>AMADYDTYVSNVQINNLSYGVYTSGGKETQFFCIGLKHGSEAISINAMCKVDVYGNHKQGFDNMLNTAKYYYTTGGDVRIYYKENVWRDPDFKSAFSSRELIAITTCSSSSYCMGPTVTN[5x];> NISDYKVMTWNLQGSSASTESKWNVNVRQLLSGTAGVDILMVQEAGAVPTSAVPTGRHIQPFGVGIPIDEYTWNLGTTSRQDIRYIYHSAIDVGARRVNLAIVSRQRADNVYVLRPTTVASRPVIGIGLGNDVFLTAHALASGGPDAAAIVRVTINFFRQPQMRHLSWFLAGDFNRSPDRLENDLMTEHLERVVAVLAPTEPTQIGGGILDYGVIVDRAPYSQRVEALRNPQLASDHYPVAFLARSCL;> VDFVYRVDSTPPDVIFRDGFSLLGYNRNFQQFISGRSCSGGSSDSRYIATTSSVNQTYAIARAYYSRSTFKGNLYRY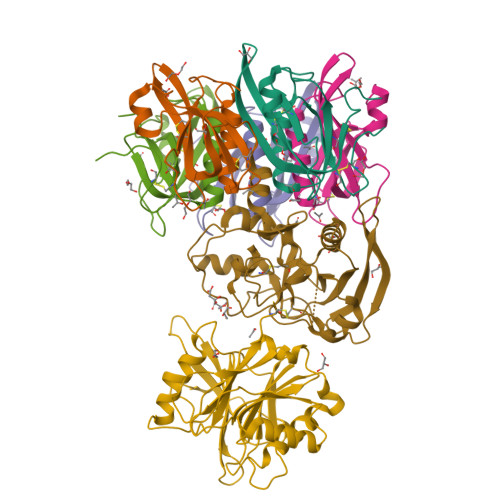QIRADNNFYSLLPSITYLETQGGHFNAYEKTMMRLQREYVSTLSILPENIQKAVALVYDSATGLVKDGVSTMNASYLGLSTTSNPGVIPFLPEPQTYTQQRIDAFGPLISSCFSIGSVCHSHRGQRADVYNMSFYDARPVIELILSK>GPRTQPAENESTPIQQLLEHFLRQLQRKDPHGFFAFPVTDAIAPGYSMIIKHPMDFGTMKDKIVANEYKSVTEFKADFKLMCDNAMTYNR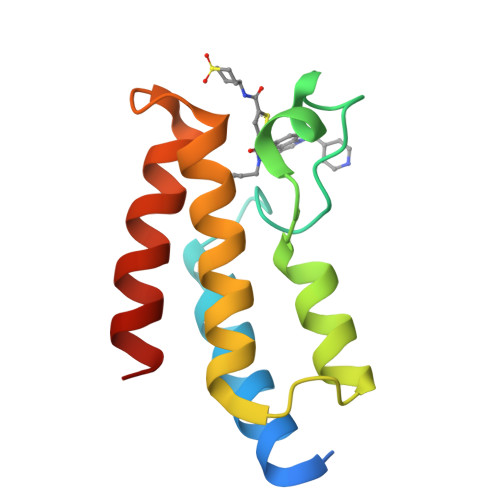PDTVYYKLAKKILHAGFKMMSKQ[2x]>ADPVRSSSRTPSDKPVAHVVANPQAEGQLQWLNRRANALLANGVELRDNQLVVPSEGLYLIYSQVLFKGQGCPSTHVLLTHTISRIAVSYQTKVNLLSAIKSPCQRETPEGAEAKPWYEPIYLGGVFQLEKGDRLSAEINRPDYLDFAESGQVYFGIIALEFRSGRLVPR[6x];>ADPLVPHLGDREKRDSVCPQGKYIHPQNNSICCTKCHKGTYLYNDCPGPGQDTDCRECESGSFTASENHLRHCLSCSKCRKEMGQVEISSCTVDRDTVCGCRKNQYRHYWSENLFQCFNCSLCLNGTVHLSCQEKQNTVCTCHAGFFLRENECVSCSNCKKSLECTKL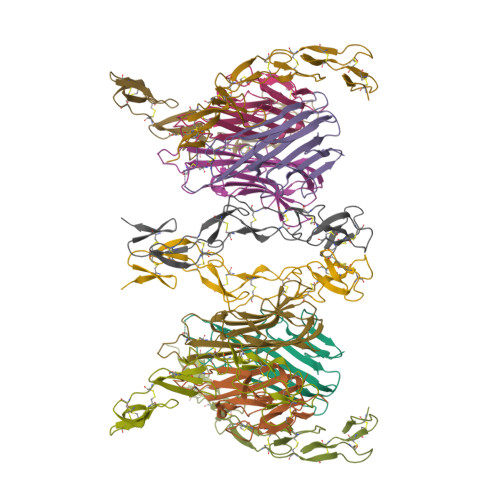CLPQIENVKGTEDSGTTGGGGSHHHHHHHH[6x]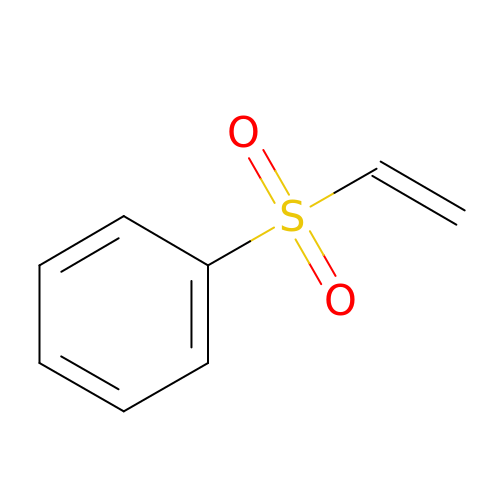(ethenylsulfonyl)benzene | C8 H8 O2 S | UJTPZISIAWDGFF-UHFFFAOYSA-N>[2x]MANDSPAKSLVDIDLSSLRDPAGIFELVEVVGNGTYGQVYKGRHVKTGQLAAIKVMDVTEDEEEEIKLEINMLKKYSHHRNIATYYGAFIKKSPPGHDDQLWLVMEFCGAGSITDLVKNTKGNTLKEDWIAYISRE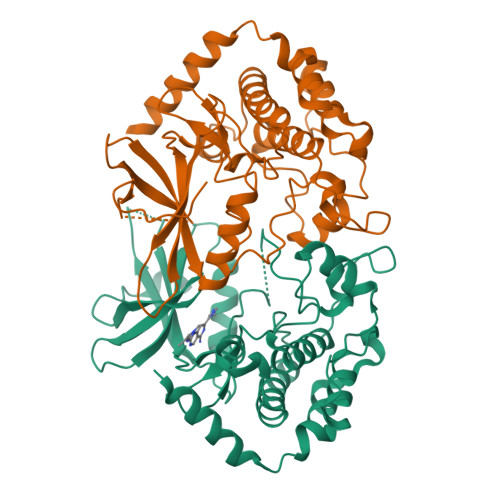ILRGLAHLHIHHVIHRDIKGQNVLLTENAEVKLVDFGVSAQLDRTVGRRNTFIGTPYWMAPEVIACDENPDATYDYRSDLWSCGITAIEMAEGAPPLCDMHPMRALFLIPRNPPPRLKSKKWSKKFFSFIEGCLVKNYMQRPSTEQLLKHPFIRDQPNERQVRIQLKDHIDRTRKKRLENLYFQ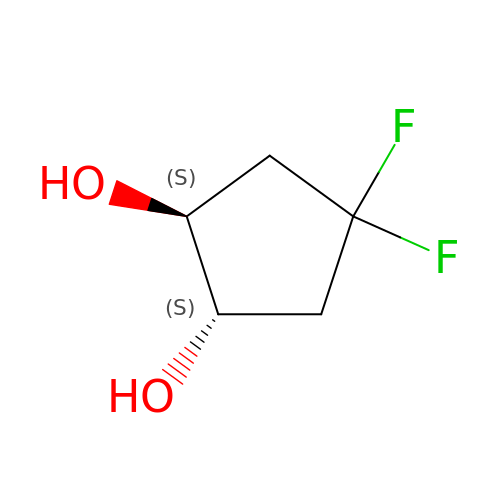trans-4,4-difluorocyclopentane-1,2-diol | C5 H8 F2 O2 | RQJNPJXCMOLSSC-IMJSIDKUSA-N>MDIEFTTSAASQASLPRGRRTARPSGDDRELAILATAENLLEDRPLADISVDDLAKGAGISRPTFYFYFPSKEAVLLTLLDRVVNQADMALQTLAENPADTDRENMWRTGINVFFETFGSHKAVTRAGQAARATSVEVAELWSTFMQKWIAYTAAVIDAERDRGAAPRTLPAHELATALNLMNERTLFASFAGEQPSVPEARVLDTLVHIWVTSIYGENRGSHHHHHH[4x]

The mycobacterial HTH-transcriptional regulator (EthR) has been reported to be a facilitator for the resistance of the second-line tuberculosis drug, ethionamide. Studies of the resistance mechanism of ethionamide revealed that an increase in the expression of HTH-Transcriptional regulator, EthR, reduces transcription and the level of active EthA protein, and results in resistance by M. tuberculosis. The discovery of this transcriptional regulator led to the notion of controlling EthA expression levels by targeting EthR and thus boosting the bactericidal effect of ethionamide. EthR binding site is characterized by a long hydrophobic tunnel surrounded mostly by hydrophobic residues, many of which are aromatic, plus four polar amino acids and a basic residue.

We then managed to obtain X-ray crystal structures for compounds 1, 2, 3, 5, 6, 7, 10, and 12 bound to EthR. Another common feature shared between several of the compounds (1, 2, 3, 7, and 10) is the presence of a ketone that forms a hydrogen bond with N176 in all but compound 3.> MASVHGTTYELLRRQGIDTVFGNPGFNELPFLKDFPEDFRYILALQEACVVGIADGYAQASRKPAFINLHSAAGTGNAMGALSNARTSHSPLIVTAGQQTRAMIGVEASETNVDAANLPRPLVKWSYEPASAAEVPHAMSRAIHMASMAPQGPVYLSVPYDDWDKDADPQSHHLFDRHVSSSVRLNDQDLDILVKALNSASNPAIVLGPDVDAANANADCVMLAERLKAPVWVAPSAPRCPFPTRHPCFRGLMPAGIAAISQLLEGHDVVLVIGAPVFRYYQYDPGQYLKPGTRLISVTCDPLEAARAPMGDAIVADIGAMASALANLVEESSRQLPTAAPEPAKVDQDAGRLHPETVFDTLNDMAPENAIYLNESTSTTAQMWQRLNMRNPGSYYFCAAGGLGFALPAAIGVQLAEPERQVIAVIGDGSANYSISALWTAAQYNIPTIFVIMNNGTYGMLRWFAGVLEAENVPGLDVPGIDFRALAK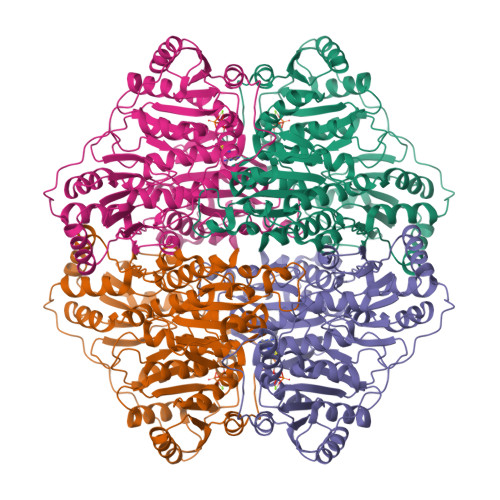GYGVQALKADNLEQLKGSLQEALSAKGPVLIEVSTVSPVK> MDPKAEGNGENITETAAGNVETSDFVNLKRQKREGVNSTGMSEIDMTGSQETPEHNMHGSPTHTDDLGPRLDADMLDSQSSHVSSSAQGNRSEVENELSNLFAKMALPGHDRRTDEYILVRQTGQDKFAGTTKCNLDHLPTKAEFNASCRLYRDGVGNYYPPPLAFERIDLPEQLAAQLHNLEPREQSKQCFQYKLEVWNRAHAEMGITGTDIFYQTDKNIKLDRNYKLRPEDRYIQTEKYGRREIQKRYEHQFQAGSLLPDILIKTPQNDIHFSYRFAGDAYANKRFEEFERAIKTKYGSDTEIKLKSKSGIMHDSKYLESWERGSA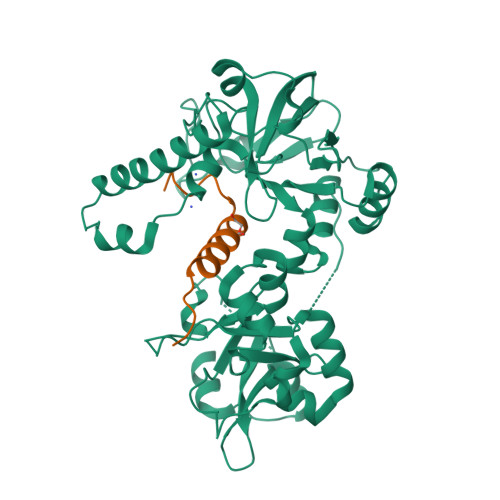DIRFAEFAGENRAHNKQFPAATVNMGRQPDGQGGMTRDRHVSVDYLLQNLPNSPWTQALKEGKLWDRVQVLARDGNRYMSPSRLEYSDPEHFTQLMDQVGLPVSMGRQSHANSVKFEQFDRQAAVIVADGPNLREVPDLSPEKLQQLSQKDVLIADRNEKGQRTGTYTNVVEYERLMMKLPSDAAQLLAEPSDRYSRAFVRPEPALPPISDSRRTYESRPRGPTVNSL;> MVIIKLNANKNMPVLAVEKPQEIHKEELSDHHQSNGFTSLDLEMIELENFVLHCPLPEENLAG> AAAAAAAAAAAAAAAAAA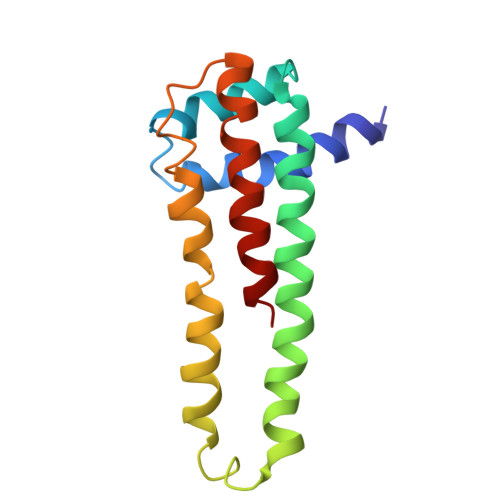AAAAAAAAAAAAAAAAAAAAAAAAAAAAAAAAAAAAAAAAAAAAAAAAAAAAAAAAAAAAAAAAAAAAAAAAAAAAAAAAAAAAAAAAAAAAAAAAAAAAAAAAAAAAAAAAAAAAAA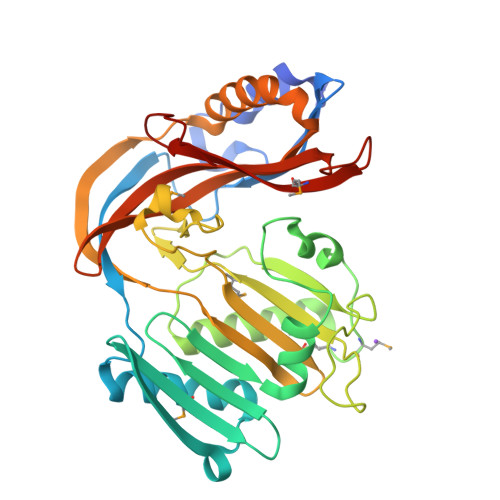> GIDDGTQANTTDLNDYENVLNSLDEEQIGKLPQNIKCVVNDKLNIDSEINIWDATSYYVKSGKVKAINFSENKDKCYDLMEKLAKAINLNKDVCVQSHRSENGNEIYLWDNNYTQDSIAIRNDSALAETHDGKLAVSASKFGTYYSPFNDKDKFRTDKQLMFMSAEEAEELAVKTAKELEINVCEKNELYVLDDKNTLIFPEDDTDKQNDTYVFFMFPDVYGIPYSRCPENEALTGYANQENHLVIAMDEKGISFLDIPPLYDWVETTETGEILHPSSILSKEVDKLKKYVTSGDIEVSEISLEYMLFADKNETYDIKPVWVVYYYQNQLVTGENSYTQKMALYDVYDAYTGEEYRIQ>[6x]MNLEKLEVSHDADSLCVVIEISKHSNIKYELDKESGALMVDRVLYG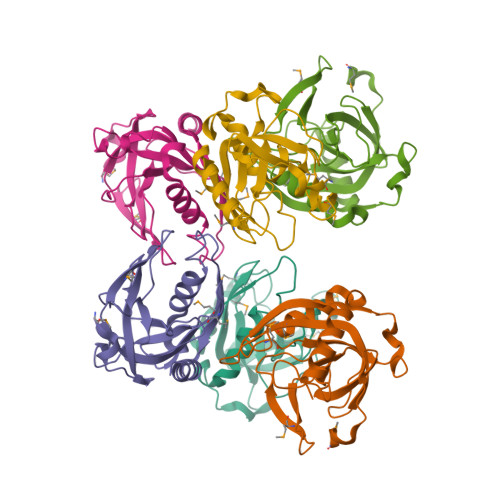AQNYPANYGFVPNTLGSDGDPVDALVLSDVAFQAGSVVKARLVGVLNMEDESGMDEKLIALPIDKIDPTHSYVKDIDDLSKHTLDKIKHFFETYKDLEPNKWVKVKGFENKESAIKVLEKAIKAYQG>[12x]MPIMGQDVKYLFQSIDAATGSAPLFPAYQTDGSVSGERELFDEQTKNGRILGPGSVADSGEVTYYGKRGDAGQKAIEDAYQNGKQIKFWR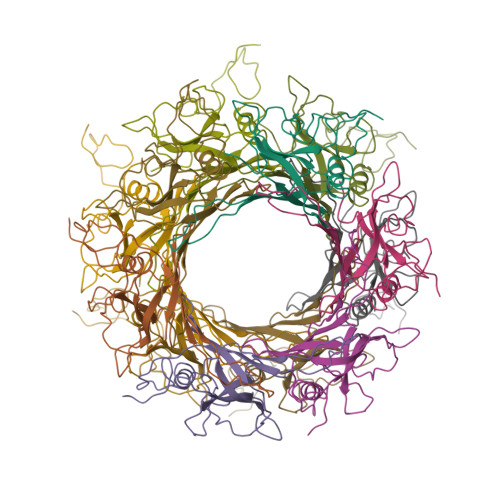VDTVKNENDKYDAQFGFAYIESREYSDGVEGAVEISISLQVIGELKNGEIDTLPEEIVNVSKGGYDFQQPGQTTGEAPGTVPAPHHHHHH> MLSTSQAFLASLRYRRPYWMLFLKGADNWKIYTVIQQPDHQRTEMLYQAWLGGLDRPYVRPKCMAHQP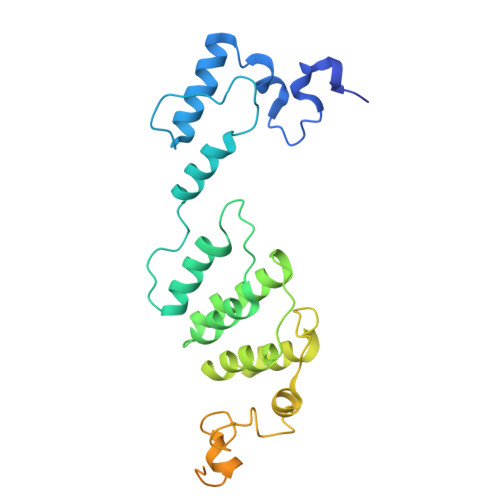VWLSKKRHLLQKARLEGPETSVEKYVLEWYKKFHSFQGTDRPTAEDLHTAFDLVERPLDLSYACQLLNQCRNHYYIRLSDDSFEIFLEACLRVDRRDCAIYALEHAEELGFWHVSDNCRRYLAGEQTWYKRSPVDLLYYPLEENAERNTAVTSGTAASAVAASDKVKGDEKVEGAPRTSATTSATAASAENEGEAEVTDDEIARLQAELEALEREIGSEGADGTDKD> ADDIVLKAKNGDVKLPHKAHQKAVPDCKKCHEKGPGKIEGFGKEMAH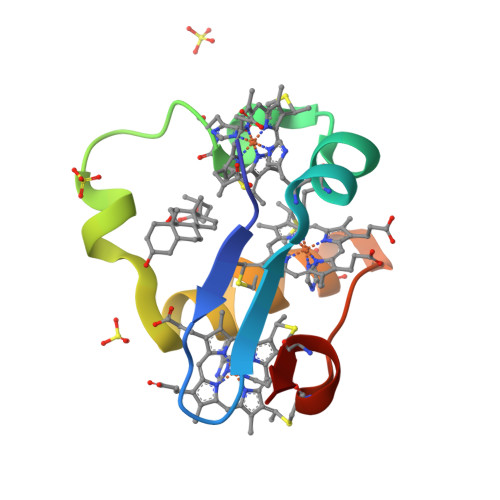GKGCKGCHEEMKKGPTKCGECHKK> MSYQSTIVPVELHSFEDAQVIGGAFRDGDAVVFDMSLLSREEARRIVDFAAGLCFALRGKM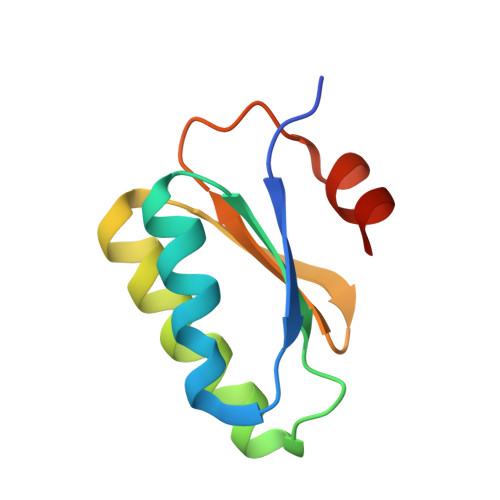QKIDSVTFAVVPELSNISTSELERAARIR>LRSSSQNSSDKPVAHVVANHQVEEQLEWLSQRANALLANGMDLKDNQ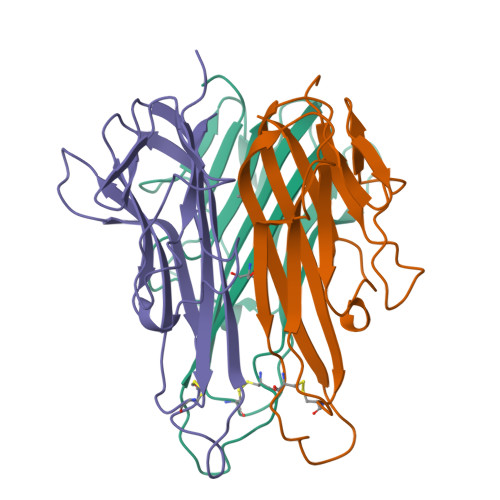LVVPADGLYLVYSQVLFKGQGCPDYVLLTHTVSRFAISYQEKVNLLSAVKSPCPKDTPEGAELKPWYEPIYLGGVFQLEKGDQLSAEVNLPKYLDFAESGQVYFGVIAL[3x]>GDITHMEKLGKLQYSLDYDFQNNQLLVGIIQA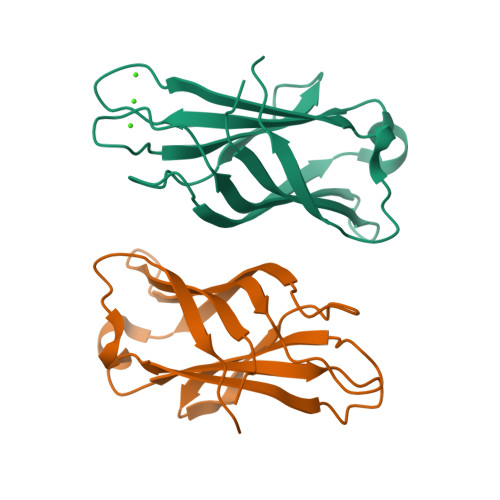AELPALDMGGTSDPFVKVFLLPDKKKKFETKVHRKTLNPVFNEQFTFKVPYSELGGKTLVMAVYDFDRFSKHDIIGEFKVPMNTVDFGHVTEEWRDLQSAE[2x]N-[(3S)-3-amino-3-carboxypropyl]-L-histidine 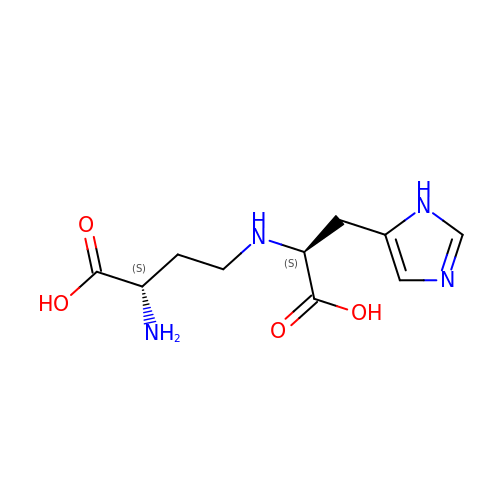| C10 H16 N4 O4 | PQUPEWJRDBYFHU-YUMQZZPRSA-N>MIKAVVF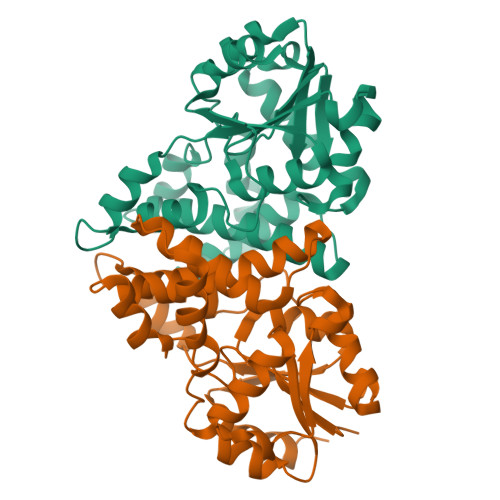DAYGTLFDVQSVADATERAYPGRGEYITQVWRQKQLEYSWLRALMGRYADFWSVTREALAYTLGTLGLEPDESFLADMAQAYNRLTPYPDAAQCLAELAPLKRAILSNGAPDMLQALVANAGLTDSFDAVISVDAKRVFKPHPDSYALVEEVLGVTPAEVLFVSSNGFDVGGAKNFGFSVARVARLSQEALARELVSGTIAPLTMFKALRMREETYAEAPDFVVPALGDLPRLVRGMAGAHLAPAV[2x]> SDLDRCTTFDDVQAPNYTQHTSSMRGVYYPDEIFRSDTLYLTQDLFLPFYSNVTGFHTINHTFDNPVIPFKDGIYFAATEKSNVVRGWVFGSTMNNKSQSVIIINNSTNVVIRACNFELCDNPFFAVSKPMGTQTHTMIFDNAFNCTFEYISDAFSLDVSEKSGNFKHLREFVFKNKDGFLYVYKGYQPIDVVRDLPSGFNTLKPIFKLPLGINITNFRAILTAFSPAQDTWGTSAAAYFVGYLKPTTFMLKYDENGTITDAVDCSQNPLAELKCSVKSHHHHHH

The key determinant of host specificity is the envelope-located trimeric spike (S) glycoprotein, which can be further cleaved by host proteases into an N-terminal S1 subunit and a membrane-bound C-terminal S2 region. In the S1 subunit, the receptor binding domain (RBD, also called the C terminal domain, CTD) is localized in the C-terminal region, spanning ∼200 amino acids, and structural studies have revealed that the RBD consists of two subdomains: the core and external subdomains. For both MERS-CoV and SARS-CoV S proteins, the S2 subunit is mainly composed of α-helices and forms the stem region of the S protein. Here we present high-resolution structures of the trimeric MERS-CoV and SARS-CoV S proteins in its pre-fusion conformation by single particle cryo-electron microscopy (cryo-EM).

To date, little is known about the structural and functional information of NTDs for the MERS-CoV or SARS-CoV S proteins, though its counterparts from other CoVs, such as mouse hepatitis virus (MHV) and bovine coronavirus (BCoV), act as receptor binding domains and their crystal structures have already been delineated. We also solved the crystal structure of the NTD at a resolution of 2.2 Å. Our crystal and cryo-EM structures show that MERS-CoV and SARS-CoV NTDs fold into galectin-like structures as in BCoV, MHV and HKU1CoV. By contrast, the NTD domain is observed with strong and clear density, forming a stable triangular platform on the top of the S trimer. The flexible RBD regions are located on the triangular edges between the NTD domains. Since the RBD is located between the NTD domains, a strategy to develop neutralizing antibodies, which target the NTD and interfering with receptor binding through steric hindrance should be feasible in the future.>[8x]MARIGIHSFVWSASSAQSELERTLANTRDAGFDLIEFSYLDPADVDIGRLAKRIADLGLGVAISIGLPADGDISSADKAVAARGVEILNQTIALTRDLGGRKVAGILSAGHGLQV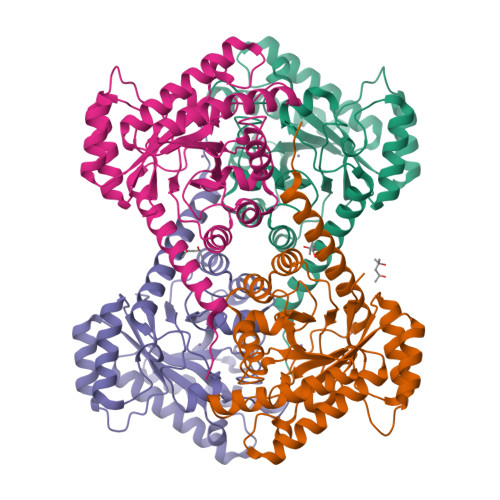EAPTRDQWNRSAAALAKVAETAKAAGVTLNLEIVNRFESNLLNTAAQGLAFIEDTGSDNIFLHLDTFHMNIEEADVGLAIRHAAGKIGYVHIGESHRGFLGTGNIDFAAIFDALTAIGYADDLSFESFSSEIVDENLSKKTAIWRNLWTDNMALAKHARAFIGLGLETARRKAELVSARHKP> L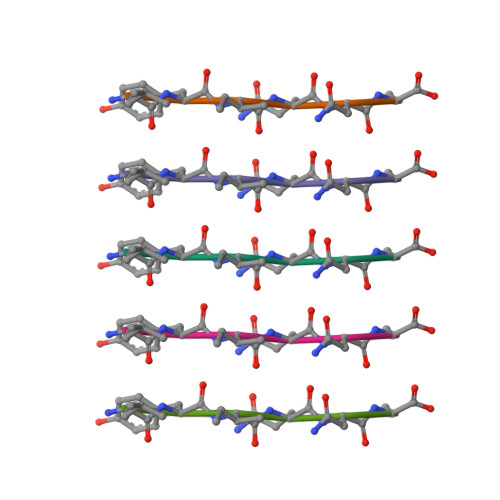YIQNL> MMQQLSLKHRLNNGDSVYGIFNSIPDPLMIEVIAASGYDFVVIDTEHV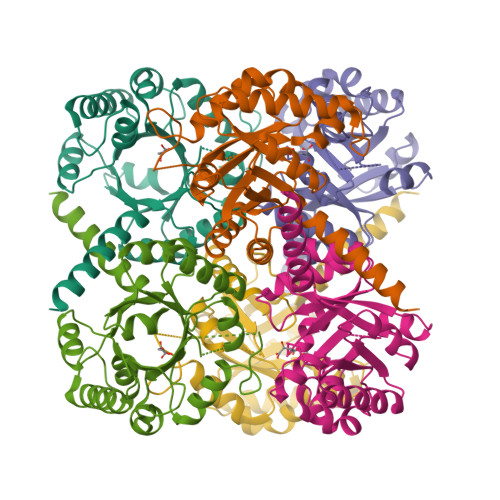AINDETLAHLIRAAEAAHIIPIVRVTAVIDRDIIKVLDMGARGIIVPHVKDRETVEHIVKLSRYYPQGLRSLNGGRMARFGRTPLLDAMEMANEHIMVIAMIQDVEGVMAIDDIAQVEGLDMIVEGAADLSQSLGIPWQTRDDQVTSHVQHIFEVVNAHGKHFCALPREDEDIAKWQAQGVQTFILGDDRGKIYRHLSASLATSKQKGDEG> SMQGPRTRPRKPIRCGEVLFAVGGWCSGDAISSVERYDPQTNEWRMVASMSKRRCGVGVSVLDDLLYA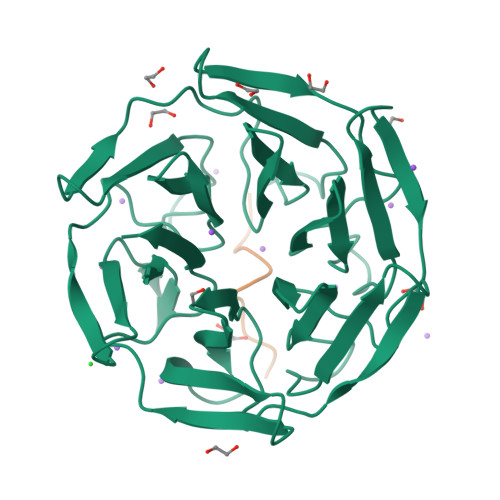VGGHDGSSYLNSVERYDPKTNQWSSDVAPTSTCRTSVGVAVLGGFLYAVGGQDGVSCLNIVERYDPKENKWTRVASMSTRRLGVAVAVLGGFLYAVGGSDGTSPLNTVERYNPQENRWHTIAPMGTRRKHLGCAVYQDMIYAVGGRDDTTELSSAERYNPRTNQWSPVVAMTSRRSGVGLAVVNGQLMAVGGFDGTTYLKTIEVFDPDANTWRLYGGMNYRRLGGGVGVIKMTHCE;> LGLPDLVAKYN(R)-1-(3-(4-amino-3-(naphthalen-1-yl)-1H-pyrazolo[3,4-d]pyrimidin-1-yl)piperidin-1-yl)prop-2-en-1-one 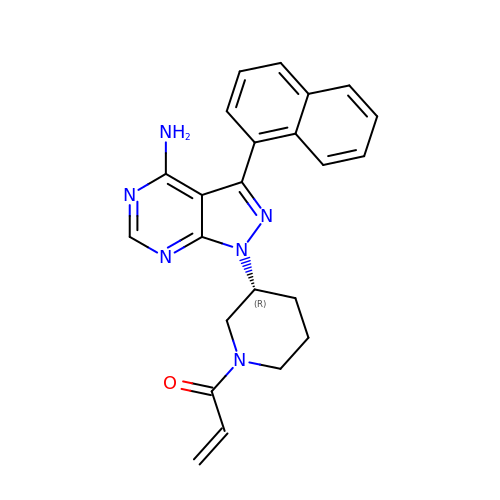| C23 H22 N6 O | WAJKANXMXJLTKT-MRXNPFEDSA-N> MMIPQTLTNTNLFIDGVSFAGDVPSLTLPKLAVKTEQYRAGGMDAPVSIDMGLEAMEAKFSTNGARREALNFFGLADQSAFNGVFRGSFKGQKGASVPVVATLRGLLKEVDPGDWKAGEKAEFKYAVAVSYYKLEVDG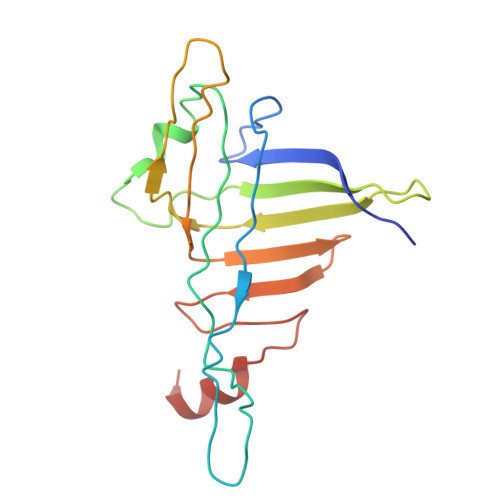REVYEIDPVNGVRAINGVDQLAGMRNDLGL> MRLDLDFGRGLVAHVMLDNVSEEQYQQISDYFVPLVNKPKLKSRDAIGQAFVMATEVCPDANPSDLWHHVLYRIYIREKIGTDPSQSWVRTSGEAFEVALVERYNPVLARHGIRLTALFKGQKGLALTRMGVADRVGSRKVDVMIEKQGGG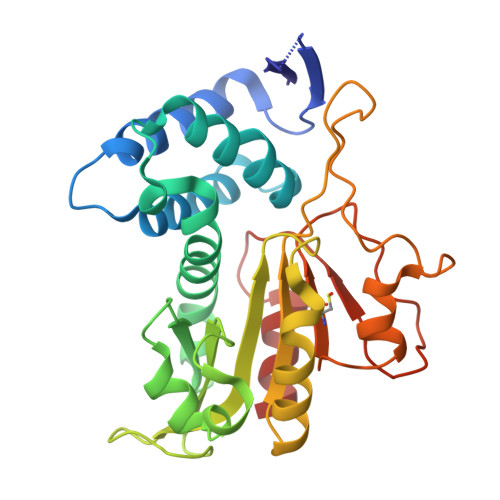RSPDAEGFGVVGGIHAKVSLAERVSDDIPASRIMMGEGLLSVLSTLDVKSFPPPHGDLVNRGELGTPDRPSDKRNYIEGHGDFSACFSYNLRTSPSNATTPSGRHIYVSGFSGQDDEFTDYLVAQLA>[4x]MKEFYLTVEQIGDSIFERYIDSNGRERTREVEYKPSLFAHCPESQATKYFDIYGKPCTRKLFANMRDASQWIKRMEDIGLEALGMDDFKLAYLSDTYNYEIKYDHTKIRVANFDIEVTSPDGFPEPSQAKHPIDAITHYDSIDDRFYVFDLLNSPYGNVEEWSIEIAAKLQEQGGDEVPSEIIDKIIYMPFDNEKELLMEYLNFWQQKTPVILTGWNVESFAIPYVYNRIKNIFGESTAKRLSPHRKTRVKVGEIITLFGISVLDYIDLYKKFSFTNQPSYSLDYISEFELNVGKLKYDGPISKLRESNHQRYISYNIIAVYRVLQIDAKRQFINLSLDMGYYAKIQIQSVFSPIKTWDAIIFNSLKEQNKVIPQGRSHPVQPYPGAFVKEPIPNRYKYVMSFDLTSLYPSIIRQVNISPETIAGTFKVAPLHDYINAVAERPSDVYSCSPNGMMYYKDRDGVV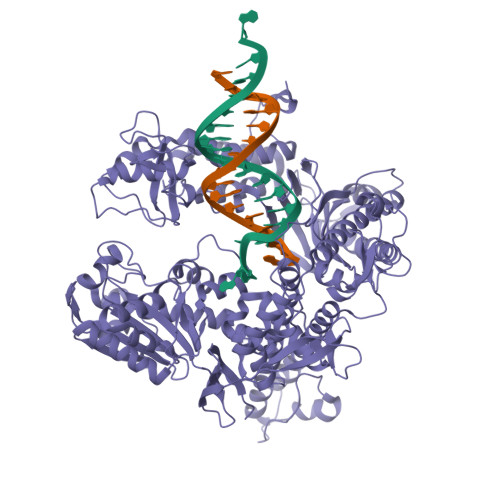PTEITKVFNQRKEHKGYMLAAQRNGEIIKEALHNPNLSVDEPLDVDYRFDFSDEIKEKIKKLSAKSLNEMLFRAQRTEVAGMTAQINRKLLINSLYGALGNVWFRYYDLRNATAITTFGQMALQWIERKVNEYLNEVCGTEGEAFVLYGDTDSIYVSADKIIDKVGESKFRDTNHWVDFLDKFARERMEPAIDRGFREMCEYMNNKQHLMFMDREAIAGPPLGSKGIGGFWTGKKRYALNVWDMEGTRYAEPKLKIMGLETQKSSTPKAVQKALKECIRRMLQEGEESLQEYFKEFEKEFRQLNYISIASVSSANNIAKYDVGGFPGPKCPFHIRGILTYNRAIKGNIDAPQVVEGEKVYVLPLREGNPFGDKCIAWPSGTEITDLIKDDVLHWMDYTVLLEKTFIKPLEGFTSAAKLDYEKKASLFDMFDF>[4x]GSMKKERVITEFWDGKIIMVSPDDPKYALKKAEEVRELVDSELGFQQVSLRCPSQTRTYMFVSNEKKIVGCLIAEPIREAYRVLAEPPSLHSLHGEPLERHRAWRCSTEPEP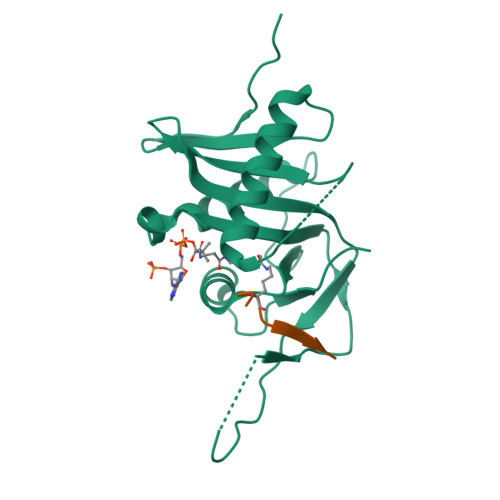AICGISRIWVFALMRRKAIASRMVDAVRSSFMYGSVLTTEEIAFSDPTPDGKLFASTYCKVPDFLVYNFVS;>[4x]RRVIGAKKDQYFL> MAHHHHHHSSGLEVLFQGPMSNDVAELKQYVLAHVSAQNASADGVLARIDDDGDGPRSWTTQWIRAGEEREQAGDLLAATTFYNMARFPFVDSPGRAEALRRCVAVFDRWRRTVPGIERLELRLPGGVVRAWAAGLSTTERRPVLLMTGGIVSIKEQWAPILPELARYGFAAVVTEMPGVGENELRYDLDSAALFGVLLDAVAERADTSRAYAMALSFSGHLALRAAPS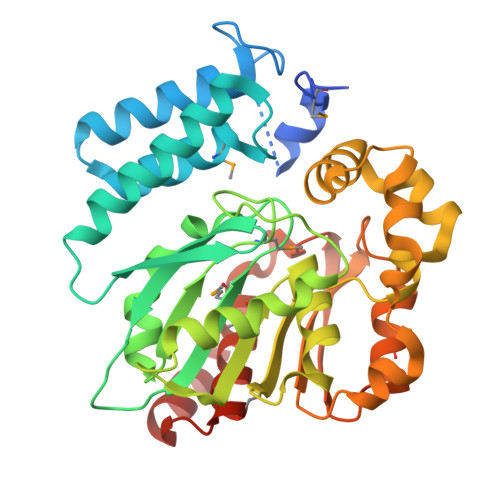EPRLRGIVTAGAPVAAFFTDKEWQAAVPRVTVDTLARLTQTTPATVFDHVRNWALTPQDLAGVRIPVAYVASGRDEIIPPADPAMLRTHVRDFRTITHDDVHGSPAHFPHTRLWTLAQVLEMSGADPRHRAAVDGALAQVEGGRA> XPWEDCAWF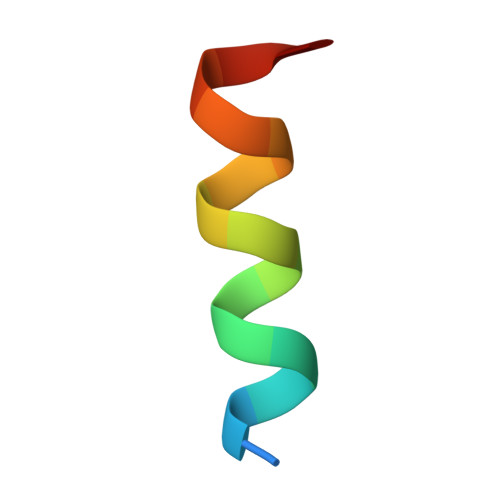AWACYNIX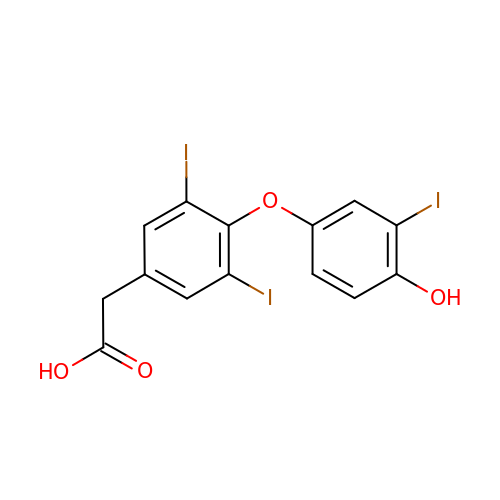[4-(4-HYDROXY-3-IODO-PHENOXY)-3,5-DIIODO-PHENYL]-ACETIC ACID | C14 H9 I3 O4 | UOWZUVNAGUAEQC-UHFFFAOYSA-N>[8x]MKITAIHLYAIRLPLRNPFVISYGSYSDMPSIIVKMETDEGIIGYGEGVADDHVTGESWESTFHTLKHTLTPALIGQNPMNIEKIHDMMDNTIYGVPTAKAAIDIACFDIMGKKLNQPVYQLIGG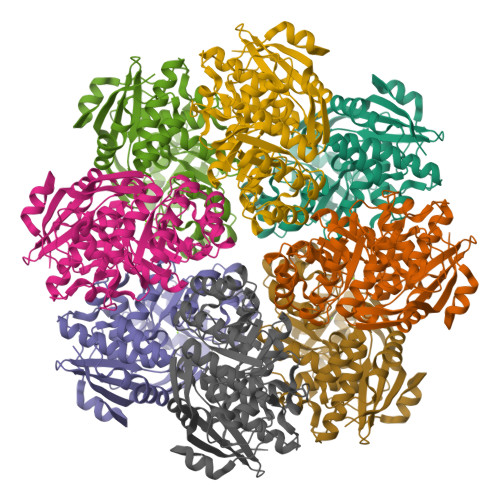RYHEEFPVTHVLSIADPENMAEEAASMIQKGYQSFKMKVGTNVKEDVKRIEAVRERVGNDIAIRVDVNQGWKNSANTLTALRSLGHLNIDWIEQPVIADDIDAMAHIRSKTDLPLMIDEGLKSSREMRQIIKLEAADKVNIKLMKCGGIYPAVKLAHQAEMAGIECQVGSMVESSVASSAGFHVAFSKKIITSVELTGPLKFTKDIGNLHYDVPFIRLNEKPGLGIEINEDTLQELTVFQDIVR>[2x]MGNYLEDCATVDVQARPTAYALAISSLGEFNSLTGGTSTDPVAEGNDYYYR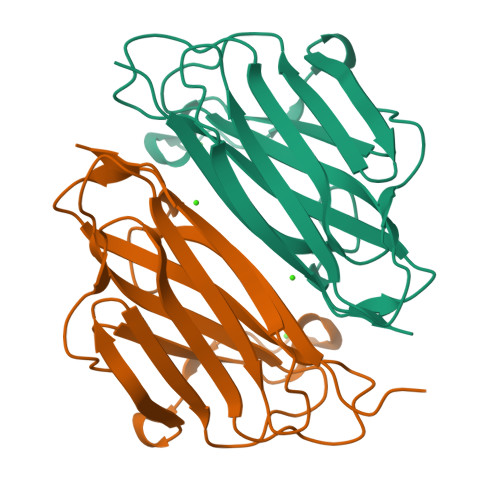FEIRAWEGSSGPQTNVTLNVTRTLGNSTFAGSGTKGVDFEVELDPDGPFGPASYAPVLSADVQVLAWGPTGVQLRYLPSLAPGATLRFSLRANAVNGTNTTVQADATSTEAPGPYTVFETTTIIP8-(2,3-dihydro-1H-inden-5-yl)-2-({4-[(3R,5S)-3,5-dimethylpiperazin-1-yl]phenyl}amino)-5-oxo-5,8-dihydropyrido[2,3-d]pyrimidine-6-carboxamide 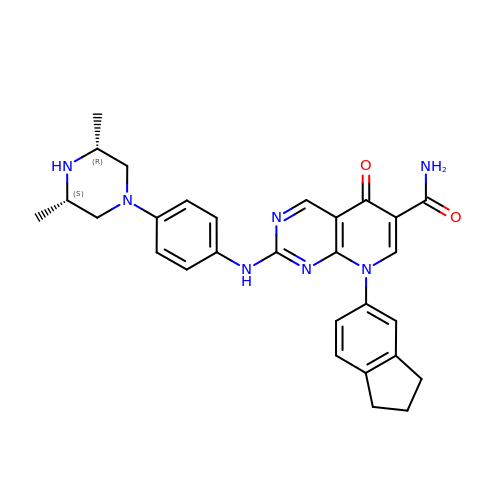| C29 H31 N7 O2 | AHBSXTVFKVCNCE-HDICACEKSA-N> MGEQVVKPTDERIIDPSTANTQLTGGVCYNTTSGGNKPLAGSPYGYETWIDTGGGVCSFCWYGA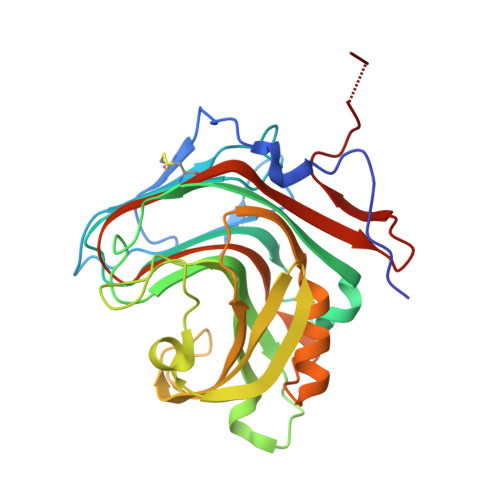DQGGGAAFKATWTNPHDFLGRLGYFWNENKPYSHYENIYCGFNYTRSGRKTAGDYSYIGIYGWSRNPSASNSNERLIEYYIVEDWFGNQWQADTSPMGINTTGGTVMGSFTVDGSSYQIIKNTRVNQPSIEGDKTFVQYFSIRQSPRKSGTISITEHFKKWEKLGMKLGDNMYECKFLIEAGAGEGFFDARLIQFYRADNEGNILQITPLEHHHHHH~{N}-[3-(5-ethanoyl-2-ethoxy-phenyl)-5-(1-methylpyrazol-3-yl)phenyl]furan-2-carboxamide | C25 H23 N3 O4 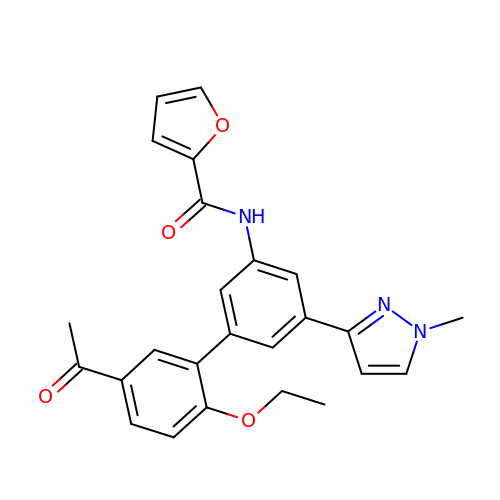| JHSSJXJMVDONGC-UHFFFAOYSA-N3-[FORMYL(HYDROXY)AMINO]PROPYLPHOSPHONIC ACID | C4 H10 N O5 P | 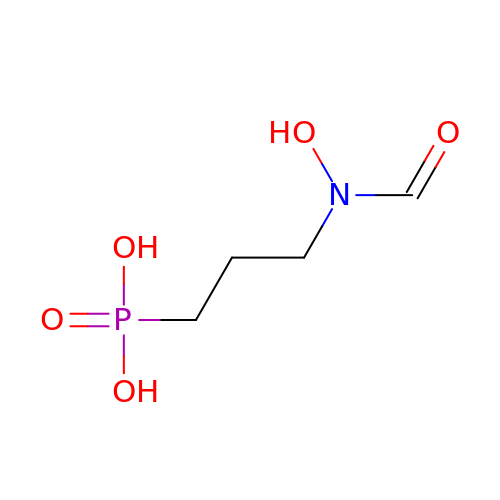GJXWDTUCERCKIX-UHFFFAOYSA-N> TLWDTTVRLSETMTLECVYPLTHNLTQVEWTKNTGTKTVSIAVYNPNHNMHIESNYLHRVHFLNSTVGFRNMSLSFYNASEADIGIYSCLFHAFPNGPWEKKIKVVWSDSFEIAAPSDSYLSAEPGQDVTLTCQLPRTWPVQQVIWEKVQPHQVDILASCNLSQETRYTSKYLRQTRSNCSQGSMKSILIIPNAMAADSGLYRCRSEAITGKNKS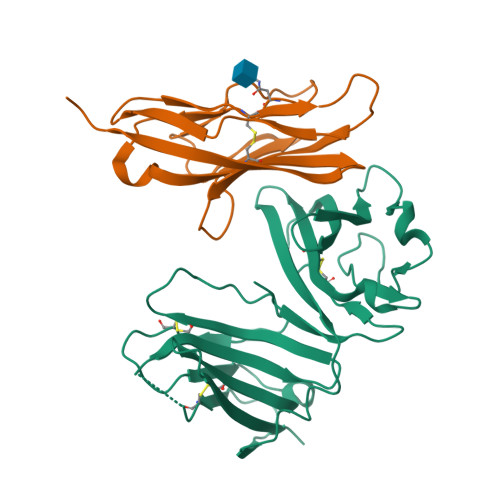FVIRLIIT;> DVVVQAPTQVPGFLGDSVTLPCYLQVPNMEVTHVSQLTWARHGESGSMAVFHQTQGPSYSESKRLEFVAARLGAELRNASLRMFGLRVEDEGNYTCLFVTFPQGSRSVDIWLRVLAKP> MIKEMIEDFISKGGLIFTHSGRYTNTNNSCFIFNKNDIGVDTKVDMYTPKSAGIKNEEGENLWQVLNKANMFYRIYSGELGEELQYLLKSCCTAKEDVTTLPQIYFKNGEGYDILVPIGNAHNLISGTEYLWEHKYYNTFTQKLGGSNPQNCTHACNKMRGGFKQFNCTPPQVEDNYNA;> MRKFIIVKNVKVDGINAKSSDITVGMPPATTFCGLGETMSIKTGIVVKAVSYGSVKFEVRGSRFNTSVTKFAWQDRGNGGKANNNSPIQPKPLADGVFTLCFEVEWEDCAEVLVDKVTNFINTARIAGGTIASFNKPFVKVAKDAEELASVKNAMMPCYVVVDCGVEVNIFEDAVNRKLQPMVNGYKKLEKIVDNKHMRDKFTPAYLATPTYTMIGYKMVSNVDNFDQALWQ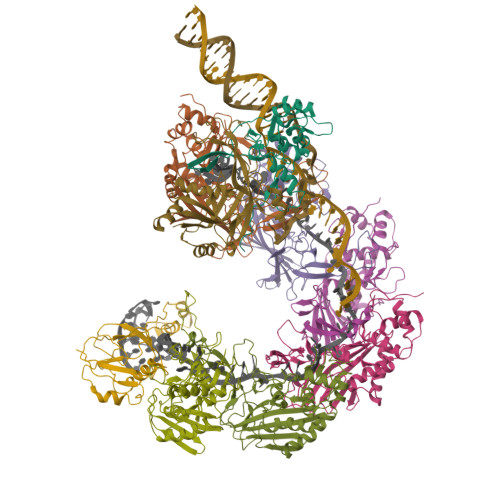YGENTKVKTIGGIYND;>MTKLKAPAVLAYSRKINPTNALMFAVNWSDRDNTTAVMVGTKTVAGTQSVRGNPNDADKGNIQTVNFANLPHNKNTLLVKYNVKFVGDVFKAELGGGEYSNTLQTALENTDFGTLAYRYVYNIAAGRTLWRNRVGAESIETVITVNDQTFTFSDLLVNEFDEDVDVAEIADMVAGVLSGEGFVTLKVEHYMLLGEGSEVFPSQEFVENSKLSKQLFDLNGQAAMHDQKIGNAIRTIDTWYEDATTPIAVEPYGSVVRNGVAYRAGNKTDLFTLMDGAVNGKSLTEEDQMFVTANLIRGGVFGGGKD[6x];> MYNTISITVVDADDVGVNFVVSKVLSTLHNKGIFNGEVGVTFPRMDKNVGDIITLFSKTGVDRKVLTSTLNTLTDFIHIGKPKEADKVKTYRKVDTKSKGKLIRRCIKRKGVSAETAESLYGNYKGEKCKLPYIVVNSKSTGQRFSMFLEECENSEKFNSYGLCIVSC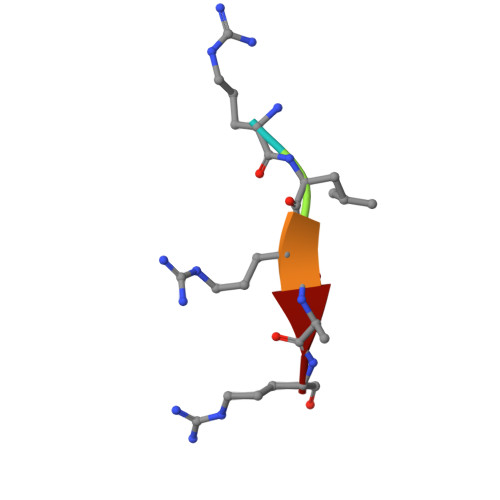> RLRAR>[2x]QKTKQFSVPNLPLNVMSNSRVPSLLNAMVVSPDQAQVVQFQNGRCTLDGQMLGTTTVSASCVARFRGKTFQAPDNRLGINLAEISGEPYHAFESPAPLGFPDFGDGDWHVTATKVTPSQLEANDPVVVGNVQPYNPQFAPHLGTL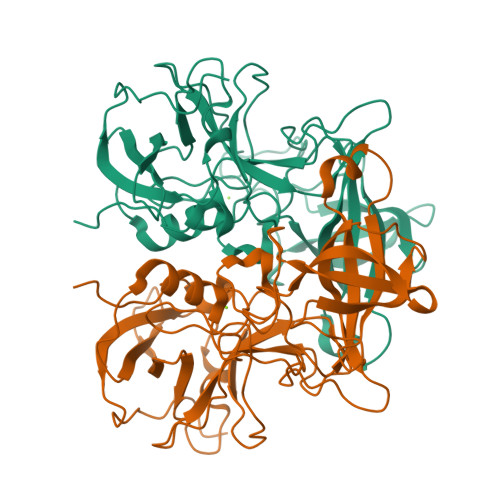VVENPTPDQVATGTDLLFNITWLSNRANNRFNPWVIPNYGSTLTEAAQLAPSIFPPGFGETIVYFNSTFPAVGATTHAAIPCLLPQEFVAHFVNEQAPIRGEAALLHYIDPDTHRNLGEFKIYPEGFVTCVPNVGGTGPQSLPTNGVFVFVSWVSRYYQLKPVGTAG>MCPQKLTISWFAIVLLVSPLMAMWELEKDVYVVEVDWTPDAPGETVNLTCDTPEEDDITWTSDQRHGVIGSGKTLTITVKEFLDAGQYTCHKGGETLSHSHLLLHKKENGIWSTEILKNFKNKTFLKCEAPNYSGRFTCSWLVQRNMDLKFNIKSSSSSPDSRAVTCGMASLSAEKVTLDQRDYEKYSVSCQEDVTCPTAEETLPIELALEARQQNKYENYSTSFFIRDIIKPDPPKNLQMKPLKNSQVEVSWEYPDSWSTPHSYFSL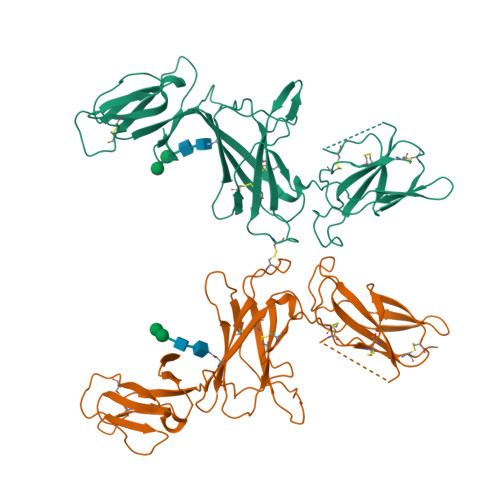KFFVRIQRKKEKMKETEEGCNQKGAFLVEKTSTEVQCKGGNVCVQAQDRYYNSSCSKWACVPCRVRSGTKHHHHHH[4x]>[4x]GMTRIASHRGGTLEFGDSTPHGFTATAAMALEEVEFDLHPTADGAIVVHHDPTL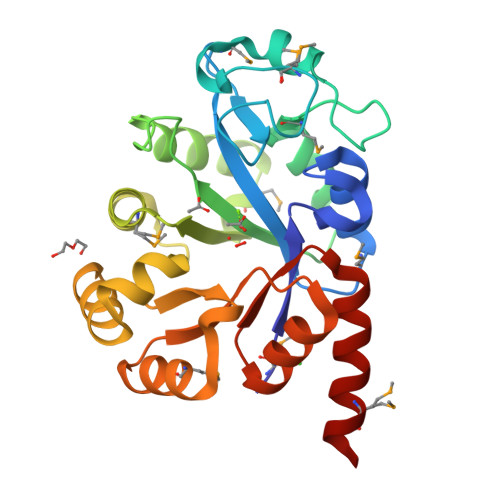DATTDMTGAIVDMTLAKVKTATIRYGAGSHPMTLEELCALYVDSHVNFRCEIKPGVDGLPYEGFVALVIAGLERHSMLERTTFSSFLLASMDELWKATTRPRLWLVSPSVLQQLGPGAVIETAIAHSIHEIGVHIDTADAGLMAQVQAAGLDFGCWAAHTPSQITKALDLGVKVFTTDRPTLAIALRTEHRMEASV> MTLELQLKHYITNLFNLPKDEKWECESIEEIADDILPDQYVRLGALSNKILQTYTYYSDTLHESN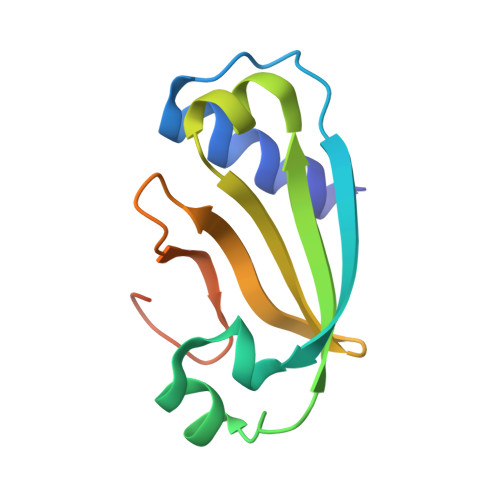IYPFILYYQKQLIAIGYIDENHDMDFLYLHNTIMPLLDQRYLLTGGQ Lysenin, the defence protein of the earthworm Eisenia fetida, is produced by coelomocytes in the body fluid that form part of the earthworm's immune system. It is a member of the aerolysin family of small β-pore-forming toxins (β-PFTs) that include key virulence factors of a large number of bacterial pathogens, such as aerolysin produced by Aeromonas spp2, Clostridium perfringens epsilon toxin3 and Clostridium septicum α-toxin4, while Bacillus thuringiensis parasporin-2 has cytocidal activity against human cancer cells. Like most PFTs, lysenin is secreted as an inactive, water-soluble monomer7. On binding to sphingomyelin (SM) in the eukaryotic cell membrane, the toxin undergoes significant changes to its secondary structure and forms oligomeric pre-pores on the membrane surface, as identified by electron crystallographic and high-speed atomic force microscopy studies, before inserting into the membrane, which leads to pore formation and consequent cell lysis.

Here we report the structure of lysenin in its nonameric membrane-inserted form determined by single particle cryo-EM, to 3.1 Å resolution. No other oligomeric species were identified during the 2D and 3D classification steps, indicating that lysenin pores are almost exclusively nonameric. Thus, each of the nine monomers in the membrane-inserted state can be divided into three domains: the N-terminal cap domain (Glu10–Ser33 and Pro108–Ile156), the β-hairpin domain (Val34–Ile107) and the C-terminal receptor-binding domain (Val157–Gly297). In contrast to the α-haemolysin family where the β-barrel begins close to the membrane-spanning region, the long β-barrel in lysenin spans the length of the assembly. The membrane-spanning region, measuring ∼35 Å, is clearly visible in filtered maps as a detergent-bound shell that delineates the boundaries of the lipid bilayer and is lined on the outside by hydrophobic residues, such as Phe, Tyr, Val and Ile. Two aromatic rings, one formed by Phe70 and the other by Tyr79 lie on the intracellular and extracellular sides of the transmembrane region, respectively. The lumen of the β-barrel is lined with charged and polar residues, including 12 threonine and 9 serine residues. Hinging on the flexible coil between Val157 and Arg159 (spheres), the N-terminal cap domain swivels downwards by ∼20 Å and rotates inwards towards the central lumen by ∼35°. The pore structure of lysenin reveals that the β-barrel recruits polypeptide from both the amphipathic loop and the two β-strands that feed into it, from here onwards referred to as the pre-insertion strands.

>[9x]MSAKAAEGYEQIEVDVVAVWKEGYVYENRGSTSVDQKITITKGMKNVNSETRTVTATHSIGSTISTGDAFEIGSVEVSYSHSHEESQVSMTETEVYESKVIEHTITIPPTSKFTRWQLNADVGGADIEYMYLIDEVTPIGGTQSIPQVITSRAKIIVGRQIILGKTEIRIKHAERKEYMTVVSRKSWPAATLGHSKLFKFVLYEDWGGFRIKTLNTMYSGYEYAYSSDQGGIYFDQGTDNPKQRWAINKSLPLRHGDVVTFMNKYFTRSGLCYDDGPATNVYCLDKREDKWILEVVGLVPRGSGHHHHHH>M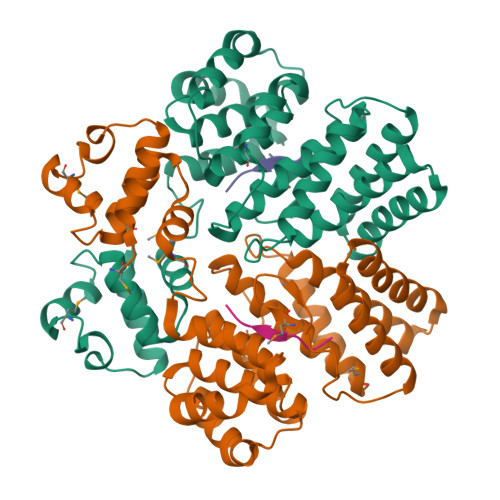FKIGSVLKQIRQELNYHQIDLYSGIMSKSVYIKVEADSRPISVEELSKFSERLGVNFFEILNRAGMNTKSVNETGKEKLLISKIFTNPDLFDKNFQRIEPKRLTSLQYFSIYLGYISIAHHYNIEVPTFNKTITSDLKHLYDKRTTFFGIDYEIVSNLLNVLPYEEVSSIIKPMYPIVDSFGKDYDLTIQTVLKNALTISIMNRNLKEAQYYINQFEHLKTIKNISINGYYDLEINYLKQIYQFLTDKNIDSYLNAVNIINIFKIIGKEDIHRSLVEELTKISAKEKFTPPKEVTMYYENYVAIENNPIPEIKEQS[4x];>[3x]LVTLVFV;> TPPKEVTM>MIELRNLTKWYPTPHGRRYVFRNLNFRFPDDVSIGLIGRNGAGKSTLMRLLGGIEAPNEGEVVTDVSISWPVGLSGGFQGSLTARENVKFVCRIYGTSHEDMLRKVRFVEEFAEIGEHFDLPMKTYSSGMRSRVAFGLSMAFDFDYYLIDEAMAVGDAQFRAKSRAVFDSRVGQANMILVSHNMNDIKEYCDVVVLVDQGQATLYEDVEAGIAAYQGSLKKAAAKPDYKDDDDK[2x];>[2x]MGKIHLAVSERSPRVKRSPWQIQQAVLFALFLRELKTRLGGRWLGVFWVLLEPVAHIAVMTTLFSLAHRAAMPSIEYPVFLITGLIPFFMFRGLVTRLMEAIDSNRGLFAYRQVKPIDTVIARAMLEISLQSIVYLIALGTLGWLGFHFLPVRALELAGVSAVLIMLGASLGLFFAVVTNEIPQARAIVRISLLPLYFVSGVIFPVHTIPPQYLPLLQLNPVLHLIELSRASFFPQYRVLQGINLAYPAGFALLSLFLALMLYRLRRHQLASVV;>MGKIHMKLVSRLTAKRLQWALVYLPMLVATVYFLVFS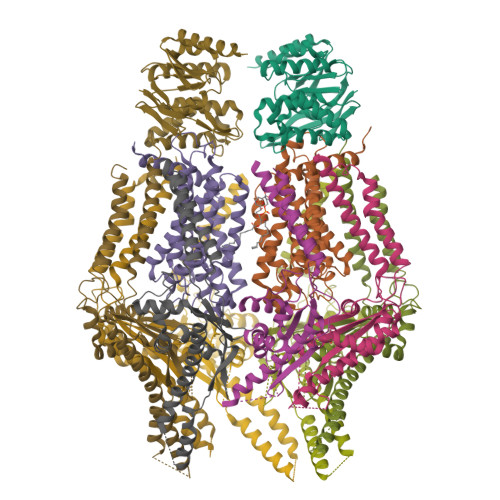ADRYVSESVITVRQTSSNAPTGGMSGAALLLAGLTPASREDTCYLQTYIHSMGLLQKLDQQLKLREHFGTPLRDPLFRLWGGTSQEWFLEYYRSRVEVLMDDICGLLTVRVQGFEPEFAQALNRAILEESERFVNELSHRMAREQGQFAEAELERATARLQEAKRQLIAFQAKHKLLDPLAQAQATGTLTAELQAALTRQEAELRNALTYLNEDSYQVKALRSQINALRQQIDEERLRATAGKNGDRINAVAAEFHDLQLQVGFAEDAYKLALAAVESARIEATRKLKSLVVVEPPVLPEIAEYPRRWYNLATLLVVCCLIYGVVSLVVATIRDHQDGSGSGSHHHHHHHHHH[8x]> MAQWIPKTAWKVSNLNKRYGAPYVAKGYASLDP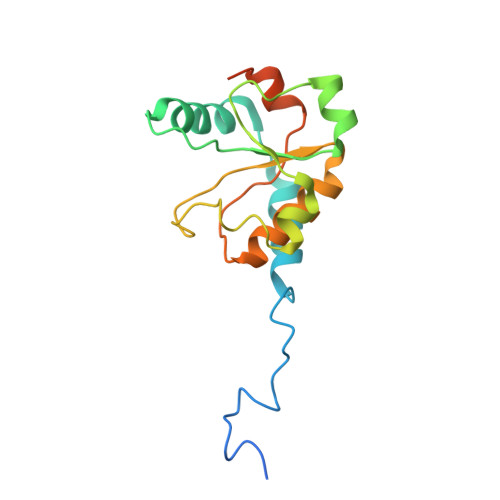RCSLDAYSSFQQTVTSADMKKALLSIDSTSSGALVIDVRSEPERRLRPLLSPAIVALHPHDILSGAACPILPSNKERAEMFVVASEAQRAVNACTALRRWGFSRVTAVSVDAVSEAIAAVQKPADAATSSSTKS> GAMGSTVDTSKLVFDGLRKKVTAMQLYECQLIDKTTLDKLLKGKKSVEEVASEIQPFLRGAGSIAGASASPKEKYSLVEAKRKKLISPESTVMLLEAQAATGGIIDPHRNEKLTVDSAIARDLIDFDDRQQIYAAEKAITGFDDPFSGKTVSVSEAIKKNLIDRETGMRLLEAQIASGGVVDPVNSVFLPKDVALARGLIDRDLYRSLNDPRDSQKNFVDPVTKKKV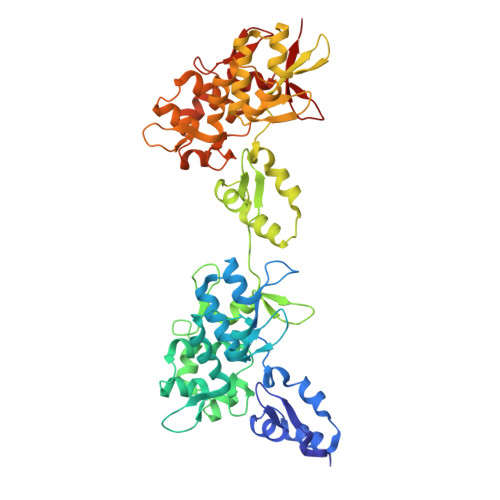SYVQLKERCRIEPHTGLLLLSVQKRSMSFQGIRQPVTVTELVDSGILRPSTVNELESGQISYDEVGERIKDFLQGSSCIAGIYNETTKQKLGIYEAMKIGLVRPGTALELLEAQAATGFIVDPVSNLRLPVEEAYKRGLVGIEFKEKLLSAERAVTGYNDPETGNIISLFQAMNKELIEKGHGIRLLEAQIATGGIIDPKESHRLPVDIAYKRGYFNEELSEILSDPSDDTKGFFDPNTEENLTYLQLKERCIKDEETGLCLLPLKE>[2x]GSHMASENDLLNKRLKLDYEEITPCLKEVTTVWEKMLSTPGRSKIKFDMEKMHSAVGQGVPRHHRGEIWKFLAEQFHLKHQFPSKQQPKDVPYKELLKQLTSQQHAILIDLGRTFPTHPYFSAQLGAGQLSLYNILKAYSLLDQEVGYC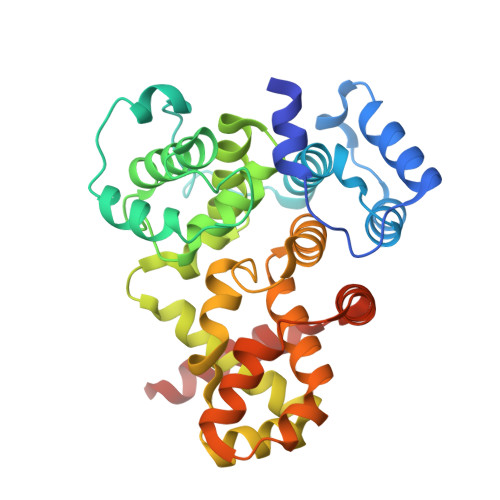QGLSFVAGILLLHMSEEEAFKMLKFLMFDMGLRKQYRPDMIILQIQMYQLSRLLHDYHRDLYNHLEEHEIGPSLYAAPWFLTMFASQFPLGFVARVFDMIFLQGTEVIFKVALSLLGSHKPLILQHENLETIVDFIKSTLPNLGLVQMEKTINQVFEMDIAKQLQAYEVEYHVLQEELIDSS>[2x]APEEERIKYVITVVEQIAKDAHRNGQEELAKLAERTAEEAKKATERGEEETLRIVYVIVVVLQIALEAHRNGQEELAKLALRTAEEAIKATERGEEETLRIVYVIVVVLQIALEAHRNGQEELAKLALRTAEEAIKATERGEEETLRIVYVIVVVLQIALEAHRNGQEELAKLALRTAEEAIKATERGEEETLRIVYVIVVVLQIALEAHRNGQEELAKLALRTAEEAIKATERGEE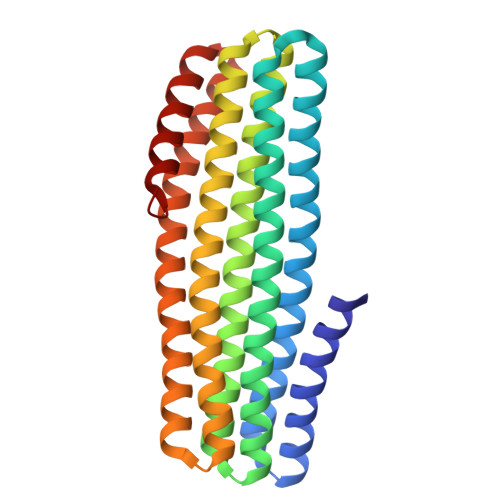ETERIVYDIVVVLQEALEAHRNGEEERAKKALDEARRRIEATERGE>TPEMPVLENRAAQGDITAPGGARRLTGDQTAALRDSLSDKPAKNIILLIGDGMGDSEITAARNYAEGAGGFFKGIDALPLTGQYTHYALNKKTGKPDYVTDSAASATAWSTGVKTYNGALGVDIHEKDHPTILEMAKAAGLATGNVSTAELQDATPAALVAHVTSRKCYGPSATSEKCPGNALEKGGKGSITEQLLNARADVTLGGGAKTFAETATAGEWQGKTLREQAQARGYQLVSDAASLNSVTEANQQKPLLGLFADGNMPVRWLGPKATYHGNIDKPAVTCTPNPQRNDSVPTLAQMTDKAIELLSKNEKGFFLQVEGASIDKQDHAANPCGQIGETVDLDEAVQRALEFAKKEGNTLVIVTADHAHASQIVAPDTKAPGLTQALNTKDGAV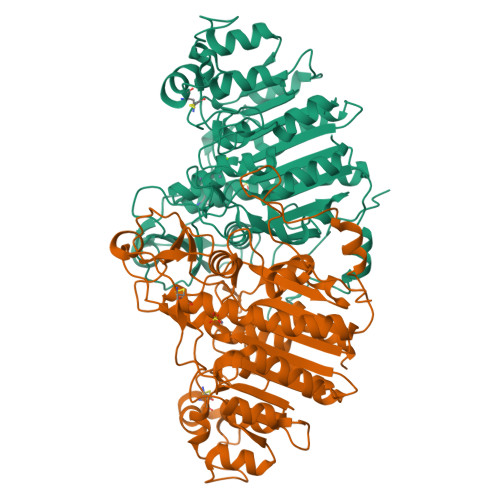MVMSYGNSEEDSQEHTGSQLRIAAYGPHAANVVGLTDQTDLFYTMKAALGLK[2x]>[2x]MNAQAEEFKKYLETNGIKPKQFHKKELIFNQWDPQEYCIFLYDGITKLTSISENGTIMNLQYY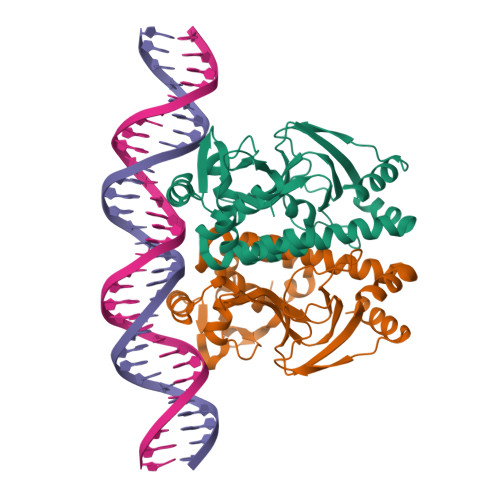KGAFVIMSGFIDTETSVGYYNLEVISEQATAYVIKINELKELLSKNLTHFFYVFQTLQKQVSYSLAKFNDFSINGKLGSICSQLLILTYVYGKETPDGIKITLDNLTMQELGYSSGIAHSSAVSRIISKLKQEKVIVYKNSCFYVQNLDYLKRYAPKLDEWFYLACPATWGKLN>[2x]MALTNAQILAVIDSWEETVGQFPVITHHVPLGGGLQGTLHCYEIPLAAPYGVGFAKNGPTRWQYKRTINQVV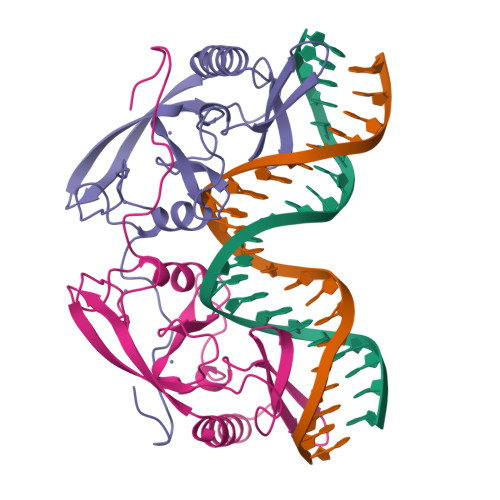HRWGSHTVPFLLEPDNINGKTCTASHLCHNTRCHNPLHLCWESLDDNKGRNWCPGPNGGCVHAVVCLRQGPLYGPGATVAGPQQRGSHFVV> MKEQLEDVLDTLTDREENVLRLRFGLDDGRTRTLEEVGKVFGVTRERIRQIEAKALRKLRHP;> MKLKILDKDNATLNVFHRNKEH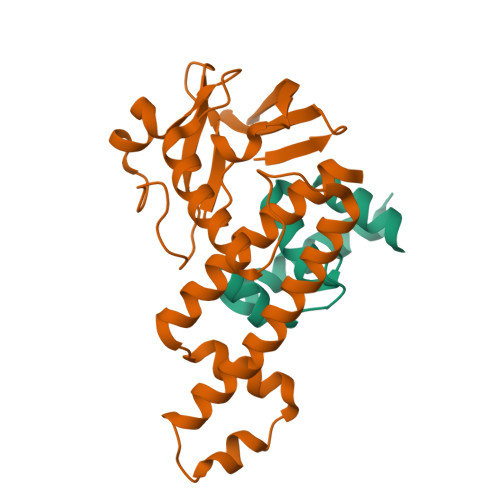KTIDNVPTANLVDWYPLSNAYEYKLSRNGEYLELKRLRSTLPSSYGLDDNNQDIIRDNNHRCKIGYWYNPAVRKDNLKIIEKAKQYGLPIITEEYDANTVEQGFRDIGVIFQSLKTIVVTRYLEGKTEEELRIFNMKSEESQLNEALKESDFSVDLTYSDLGQIYNMLLLMKKISK> SIDEVGALSKFAASLADQMRAGSNSLDRDVQSLFGVWKGSAADAYRSGWDEMQDGATKVWNALTDIASTLGS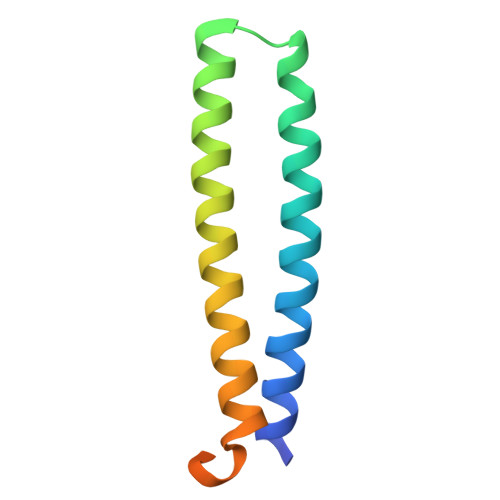NAAAFHAQETSTASSITSTQAD>[2x]MTTKISRRTFFVGGTALTALVVANLPRRASAQSRTINLYSSRHYNTDDALYDAFGEVNLIEASAEELIERIQSEGANSP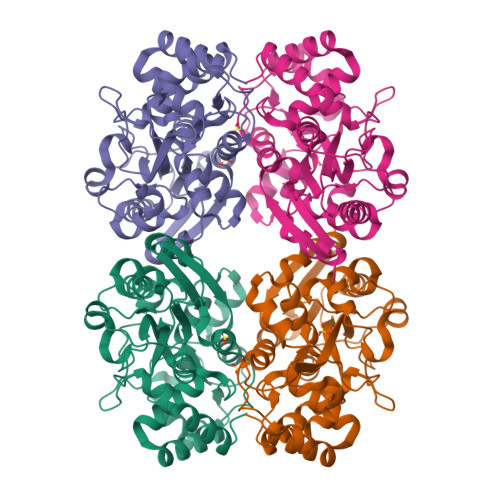GDILFTVDAGMLWRAEQAGLFQPVRSGKLNERIPENLRHPDGLWYGFTQRARVLYYSRDRVNPADLSTYEALADPQWRGKILVRPSSNVYNLSLTASRIAIHGEPETRRWLQGLVGNFARQPEGNDTAQIRAIAAGIGDVAIANSYYYIRLQKSTDPADQEVVEKVSLFFPNTGSGERGTHVNVSGAGVLKNAPNRDAAIAFLEYLASDDAQRYFAEGNNEYPVIPGVPIDPVLAAHGQLKGDPLNVSNLGRYQPDSARLMNEVGWQ> MGDSILSQAE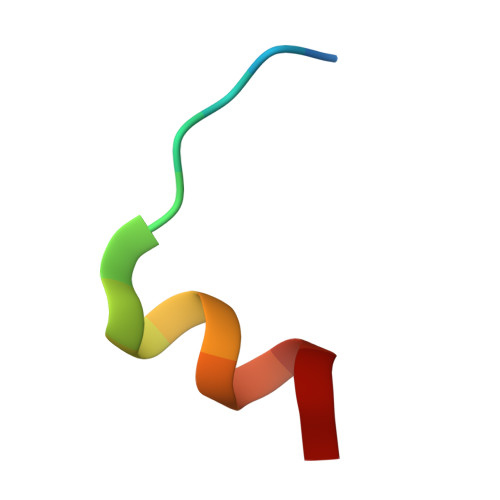IDALLN>[2x]AKNIKKGPAPFYPLEDGTAGEQLHKAMKRYALVPGTIAFTDAHIEVNITYAEYFEMSVRLAEAMKRYGLNTNHRIVVCSENSLQFFMPVLGALFIGVAVAPANDIYNERELLNSMNISQPTVVFVSKKGLQKILNVQKKLPIIQKIIIMDSKTDYQGFQSMYTFVTSHLPPGFNEYDFVPESFDRDKTIALIMNSSGSTGLPKGVALPHRTACVRFSHARDPIFGNQIIPDTAILSVVPFHHGFGMFTTLGYLICGFRVVLMYRFEEELFLRSLQDYKIQSALLVPTLFSFFAKSTLIDKYDLSNLHEIASGGAPLSKEVGEAVAKRFHLPGIRQGY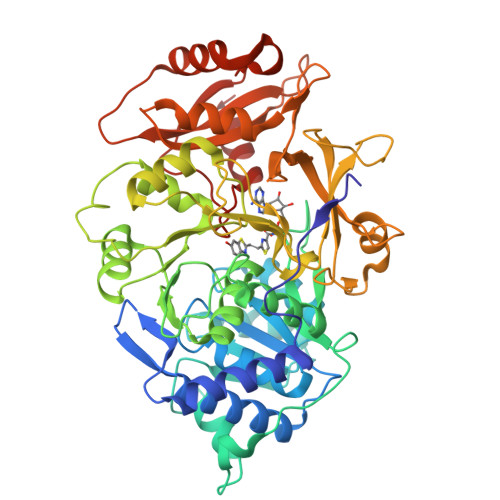GLTETTSAILITPEGDDKPGAVGKVVPFFEAKVVDLDTGKTLGVNQRGELCVRGPMIMSGYVNNPEATNALIDKDGWLHSGDIAYWDEDEHFFIVDRLKSLIKYKGYQVAPAELESILLQHPNIFDAGVAGLPDDDAGELPAAVVVLEHGKTMTEKEIVDYVASQVTTAKKLRGGVVFVDEVPKGLTGKLDARKIREILIKAKKGG> MCKDKNEKKNYEHVNANEKNGYLASEKNELTKNKVEEHTYDYDYVVIGGGPGGMASAKEAAAHGARVLLFDYVKPSSQGTKWGIGGTCVNVGCVPKKLMHYAGHMGSIFKLDSKAYGWKFDNLKHDWKKLVTTVQSHIRSLNFSYMTGLRSSKVKYINGLAKLKDKNT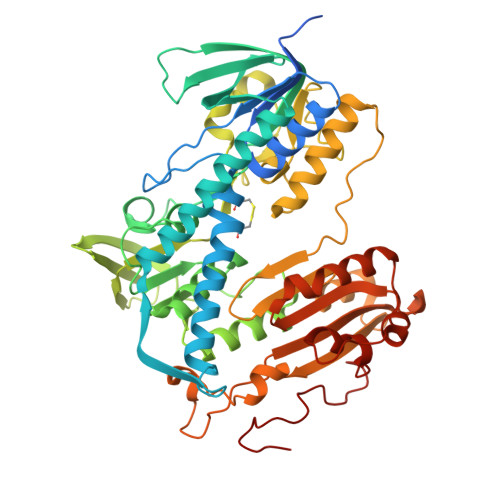VSYYLKGDLSKEETVTGKYILIATGCRPHIPDDVEGAKELSITSDDIFSLKKDPGKTLVVGASYVALECSGFLNSLGYDVTVAVRSIVLRGFDQQCAVKVKLYMEEQGVMFKNGILPKKLTKMDDKILVEFSDKTSELYDTVLYAIGRKGDIDGLNLESLNMNVNKSNNKIIADHLSCTNIPSIFAVGDVAENVPELAPVAIKAGEILARRLFKDSDEIMDYSYIPTSIYTPIEYGACGYSEEKAYELYGKSNVEVFLQEFNNLEISAVHRQKHIRAQKDEYDLDVSSTCLAKLVCLKNEDNRVIGFHYVGPNAGEVTQGMALALRLKVKKKDFDNCIGIHPTDAESFMNLFVTISSGLSYAAKGGSGGGKCG A prominent member of the PspA family is the vesicle-inducing protein in plastids 1 (Vipp1), also known as IM30 (inner membrane-associated protein of 30 kDa). Vesicle-inducing protein in plastids 1 (Vipp1) is critical for thylakoid membrane biogenesis and maintenance. Vipp1 appears to have two functions: in membrane maintenance (that is, during heat or light stress) and in thylakoid membrane (TM) biogenesis and/or remodeling. Vipp1 binds to negatively charged membranes and membrane binding depends on stored curvature elastic stress.

Using single-particle-based helical reconstruction, we resolved the structures of type I tubes at 5.1-Å resolution and two structures of type II tubes at 7.0-Å and 7.1-Å resolution. The type I and II tubes differ in their diameter and the arrangement of the monomers relative to the tube axis, as well as the diameter and thickness of the engulfed lipid bilayer tube. In contrast to the Vipp1 rings, the monomer orientation of the α1−α3 hairpin with respect to the tube axis is the same over the whole length of the tubes. Nevertheless, the monomer orientation among the tubes differs; in type I tubes, the α1−α3 hairpins are oriented parallel to the tube axis, while, in type II tubes, the hairpins are tilted approximately 45° relative to the tube axis. Remarkably, from rings over type II tubes to type I tubes, the α1−α3 hairpins accommodate a wide range of orientations along the tubulated membrane axis from perpendicular to parallel (from 90° to 0°) while essentially maintaining the same intermolecular contacts to stabilize the assembly. The here-determined structures of Vipp1 polymers in the presence of membranes indicated that helix α0 is immersed in the outer lipid leaflet of the bilayer. However, in contrast to SynPspA helix α0 that protrudes toward the bilayer, Vipp1 α0 lies flat in the membrane plane and appears to be partially submerged into the outer bilayer leaflet. The bilayer thickness in all three Vipp1 tubes remained nearly identical at 35 Å, although the inner leaflet radius changed with the tube diameter. Nevertheless, the same or similar intermolecular interactions of α0 with another α0 and α1 + α4, as observed previously in Vipp1 rings, are present in type I and II tubes.

> ALFDRLGRVVRANLNDLVSKAEDPEKVLEQAVIDMQEDLVQLRQAVARTIAEEKRTEQRLNQDTQEAKKWEDRAKLALTNGEENLAREALARKKSLTDTAAAYQTQLAQQRTMSENLRRNLAALEAKISEAKTKKNMLQARAKAAKANAELQQTLGGLGTSSATSAFERMENKVLDMEATSQAAGELAGFGIENQFAQLEASSGVEDELAALKAS> SHEQFRAALQLVVDPGDPRSYLDNFIKIGEGSTGIVCIATVRSSGKLVAVKKMDLRKQQRRELLFNEVVIMRDYQHENVVEMYN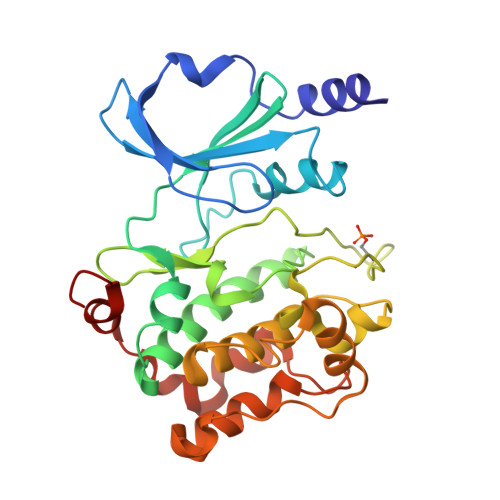SYLVGDELWVVMEFLEGGALTDIVTHTRMNEEQIAAVCLAVLQALSVLHAQGVIHRDIKSDSILLTHDGRVKLSDFGFCAQVSKEVPRRKSLVGTPYWMAPELISRLPYGPEVDIWSLGIMVIEMVDGEPPYFNEPPLKAMKMIRDNLPPRLKNLHKVSPSLKGFLDRLLVRDPAQRATAAELLKHPFLAKAGPPASIVPLMRQNRTR;> PRQWQSLIEESARRPKPLVDPACIT>MAHHHHHHDEVDMPGTKRFQHVIETPEPGKWELSGYEAAVPITEKSNPLTQDLDKADAENIVRLLGQCDAEIFQEEGQALSTYQRLYSESILTTMVQVAGKVQEVLKEPDGGLVVLSGGGTSGRMAFLMSVSFNQLMKGLGQKPLYTYLIAGGDRSVVASREGTEDSALHGIEELKKVAAGKKRVIVIGISVGLSAPFVAGQMDCCMNNTAVFLPVLVGFNPVSMARNDPIEDWSSTFRQVAERMQKMQEKQKAFVLNPAIGPEGLSGSSRMKGGSATKILLETLLLAAHKTVDQGIAASQRCLLEILRTFERAHQVTYSQSPKIATLMKSVSTSLEKKGHVYLVGWQTLGIIAIMDGVECIHTFGADFRDVRGFLIGDHSDMFNQKAELTNQGPQFTFSQEDFLTSILPSLTEIDTVVFIFTLDDNLTEVQTIVEQVKEKTNHIQALAHSTVGQTLPIPLKKLFPSIISITWPLLFFEYEGNFIQKFQRELSTKWVLNTVSTGAHVLLGKILQNHMLDLRISNSKLFWRALAM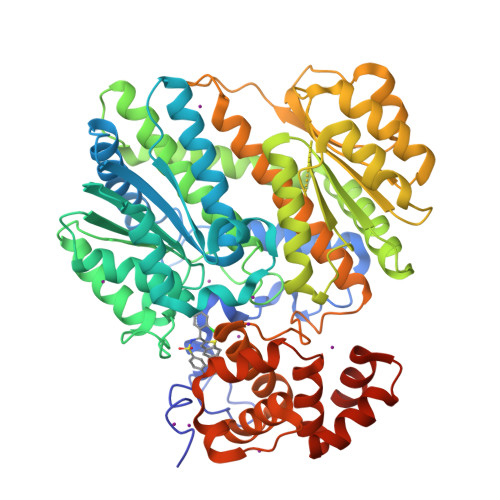LQRFSGQSKARCIESLLRAIHFPQPLSDDIRAAPISCHVQVAHEKEQVIPIALLSLLFRCSITEAQAHLAAAPSVCEAVRSALAGPGQKRTADPLEILEPDVQG[2x]>MSALLASSFVSRVAAFKAQKVQNKSVSTTVKADIYPEFGTYPGGGESPIIPFGSEKNAEREVIHGRWAMLGVTGAWAAENGTGIPWFTAGTLCTPDDCTAVADKFPGAVAPLAPEGSGYPSFWNVLIIEIVLVGAAEAYRTGISDSPFDDGLTVGDVNPGGRFDPLGLAESGDLEELKIKELKHCRLSMFAWLGCIFQALATQEGPIANWQSHVADPVHSNVLTNAAKGFGFY[2x];> XRRTKASVPAKRSAFKANKFGSLAPPDLYPEFGTYPGGGESPVIPFGSEKNAEREIIHGRWAMLGVTGAWAAENGTGIPWFTAGTLCTPDDCTAVADKFPGAVAPLAPAGSGYPNFWAVLAIEIFLVGSAECYRTGLFENPFPELTQGDVTPGGRFDPLGFAEAGDLEELKIKELKHSRLAMFAWLGCIMQALATQEGPIANWTAHVADPIHANVLTNAAKGFKFY

Here, we report the structure and function of the O. tauri photosystem I (PSI) supercomplex in low light conditions, where it expands its photon-absorbing capacity by assembling with the light-harvesting complexes I (LHCI) and a prasinophyte-specific light-harvesting complex (Lhcp). Interestingly, nine Lhcp subunits, including one Lhcp1 monomer with a phosphorylated amino-terminal threonine and eight Lhcp2 monomers, oligomerize into three trimers and associate with PSI on the third side between Lhca6 and PsaK. While Lhcp, Lhcb (apoproteins of LHCII), and Lhca (apoproteins of LHCI) all belong to the LHC superfamily, Lhcp proteins form a separate clade with characteristics of an ancestral state of LHC proteins instead of belonging to the clades of Lhcb or Lhca. In terms of pigment composition, OtLhcp1 and OtLhcp2 each contain 14 Chl molecules (8 Chl a, 5 Chl b, and 1 Mdp) and 7 carotenoid molecules (4 Dlt, 2 Prx, and 1 Nex).

Among the three trimers associated with OtPSI, Trimers 1 and 3 are both (Lhcp2)3 homotrimers, whereas Trimer 2 is a Lhcp1(Lhcp2)2 heterotrimer. Trimers 1 and 3 bind to PSI on the PsaO and PsaK sides, respectively, while Trimer 2 assembles with PSI on the PsaL-PsaH side through Lhcp1 subunit and interacts with Lhca6 through an Lhcp2 subunit. Trimer 2 binds to PSI on three different sites. At site 1, Lhcp1Trimer2 has its elongated N-terminal region (NTR) partially inserted into a surface pocket formed by PsaL and PsaH subunits. The NTR of Lhcp1 contains an RRpT (pT, phosphorylated Thr residue) motif identical to those found in Z. mays pLhcb2 and C. reinhardtii pLhcbM1. The RRpT motif of Lhcp1 interacts with nearby amino acid residues through salt bridges and hydrogen bonds, in a similar way as those of Z. mays pLhcb2 and C. reinhardtii pLhcbM1. Arg29 in Lhcp1 might be acetylated on its main-chain amine group as there is an extra density linked to it, and the van der Waals interactions between the putative acetyl group and nearby amino acid residues from PsaH serve to stabilize the association between Lhcp1 and the PSI core. Sites 2 and 3 are located in the membrane-embedded regions on the stromal and lumenal sides, respectively. On these two sites, Lhcp1 forms hydrogen bonds and van der Waals interactions with nearby amino acid residues and pigment molecules from PsaH and PsaL subunits. The Chls in Trimer 2 and Trimer 3 form multiple interfacial pairs with the Chls from Lhca6/PsaH and PsaK, respectively, which are likely to help provide the excitation energy for PSI.> GAFLDKPKMEKHNAQGQGNGLRYGLSSMQGWRVEMEAAHTAVIGLPSGLESWSFFAVYDGHAGSQVAKYCCEHLLDHITNNQDFKGSAGAPSVENVKNGIRTGFLEIDEHMRVMSEKKHGADRSGSTAVGVLISPQHTYFINCGDSRGLLCRNRKVHFFTQDHKPSNPLEKERIQNAGGSVMIQRVNGSLAVSRALGDFDYKCVHGKGPTEQLVSPEPEVHDIERSEEDDQFIILACDGIWDVMGNEELCDFVRSRLEVTDDLEKVCNEVVDTCLYKGSRDNMSVILICFPNAPKVSPEAVKKEAELDKYLECRVEEIIKKQGEGVPDLVHVMRTLASENI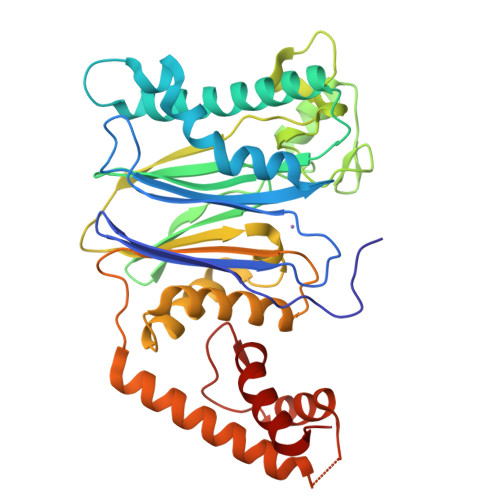PSLPPGGELASKRNVIEAVYNRLNPY>MDLSAASHRIPLSDGNSIPIIGLGTYSEPKSTPKGACATSVKVAIDTGYRHIDGAYIYQNEHEVGEAIREKIAEGKVRREDIFYCGKLWATNHVPEMVRPTLERTLRVLQLDYVDLYIIEVPMAFKPGDEIYPRDENGKWLYHKSNLCATWEAMEACKDAGLVKSLGVSNFNRRQLELILNKPGLKHKPVS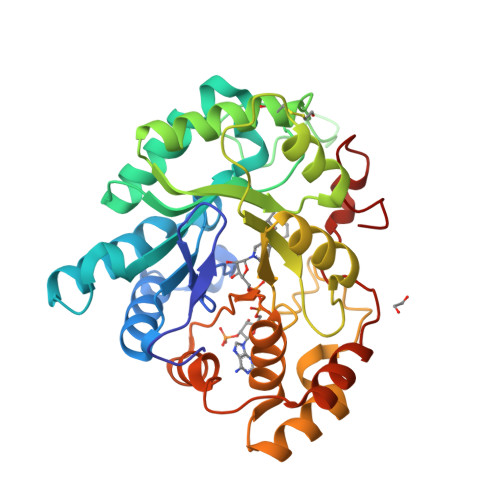NQVECHPYFTQPKLLKFCQQHDIVITAYSPLGTSRNPIWVNVSSPPLLKDALLNSLGKRYNKTAAQIVLRFNIQRGVVVIPKSFNLERIKENFQIFDFSLTEEEMKDIEALNKNVRFVELLMWRDHPEYPFHDEY[2x]> GGGRNIFTSPYKETRVNPRALEYWVSGEIHGLVDNESVSEFKEIIEGGLGILRQESEDYVARRFEVYATFNNIIPILTTKNVNEVDQKFNILIVNIESIIEICIPHLQIAQDTLLSSSEKKNPFVIRLYVQIVRFFSAIMSNFKIVKWLTKRPDLVNKLKVIYRWTTGALRNENSNKIIITAQVSFLRDEKFGTFFLSNEEIKPIISTFTEIMEINSHNLIYEKLLLIRGFLSKYPKLMIETVTSWLPGEVLPRIIIGDEIYSMKILITSIVVLLELLKKCLDFVDEHERIYQCIMLSPVCETIPEKFLSKLPLNSYDSANLDKVTIGHLLTQQIKNYIVVKNDNKIAMDLWLSMTGLLYDSGKRVYDLTSESNKVWFDLNNLCFINNHPKTRLMSIKVWRIITYCICTKISQKNQEGNKSLLSLLRTPFQMTLPYVNDPSAREGIIYHLLGVVYTAFTSNKNLSTDMFELFWDHLITPIYEDYVFKYDSIHLQNVLFTVLHLLIGGKNADVALERKYKKHIHPMSVIASEGVKLKDISSLPPQIIKREYDKIMKVVFQAVEVAISNVNLAHDLILTSLKHLPEDRKDQTHLESFSSLILKVTQNNKDTPIFRDFFGAVTSSFVYTFLDLFLRKNDSSLVNFNIQISKVGISQGNMTLDLLKDVIRKARNETSEFLIIEKFLELDDKKTEVYAQNWVGSTLLPPNISFREFQSLANIVNKVPNENSIENFLDLC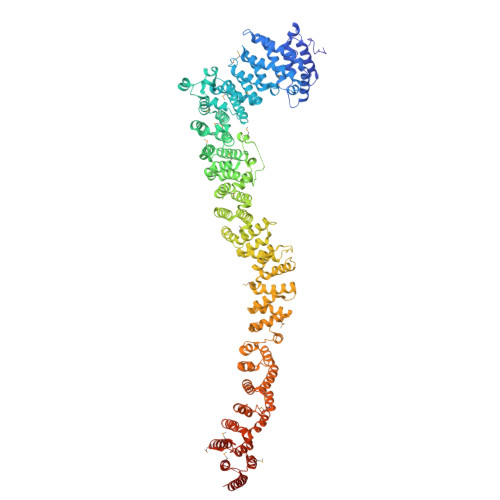LKLSFPVNLFTLLHVSMWSNNNFIYFIQSYVSKNENKLNVDLITLLKTSLPGNPELFSGLLPFLRRNKFMDILEYCIHSNPNLLNSIPDLNSDLLLKLLPRSRASYFAANIKLFKCSEQLTLVRWLLKGQQLEQLNQNFSEIENVLQNASDSELEKSEIIRELLHLAMANPIEPLFSGLLNFCIKNNMADHLDEFCGNMTSEVLFKISPELLLKLLTYKEKPNGKLLAAVIEKIENGDDDYILELLEKIIIQKEIQILEKLKEPLLVFFLNPVSSNMQKHKKSTNMLRELVLLYLTKPLSRSAAKKFFSMLISILPPNPNYQTIDMVNLLIDLIKSHNRKFKDKRTYNATLKTIGKWIQESGVVHQGDSSKEIEAI>MGFLDGKRILLTGLLSNRSIAYGIAKACKREGAELAFTYVGDRFKDRITEFAAEFGSELVF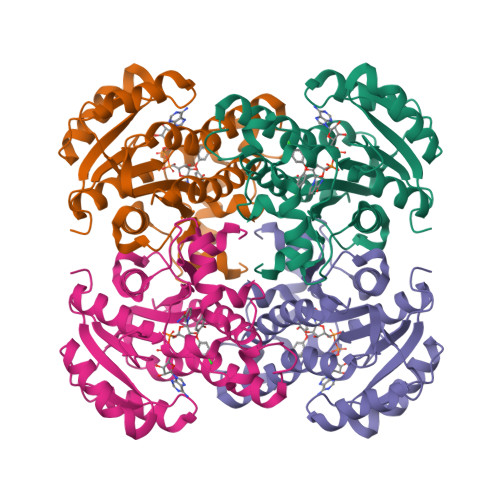PCDVADDAQIDALFASLKTHWDSLDGLVHSIGFAPREAIAGDFLDGLTRENFRIAHDISAYSFPALAKAALPMLSDDASLLTLSYLGAERAIPNYNTMGLAKAALEASVRYLAVSLGAKGVRVNAISAGPIKTLAASGIKSFGKILDFVESNSPLKRNVTIEQVGNAGAFLLSDLASGVTAEVMHVDSGFNAVVGGMAGLEEKLAAALEHHHHHH[16x]>[3x]MTWHILGAGSLGSLWAARLGRAGLPVRLILRDRQRLRRYQQAGGLSLVEDGQASLYPIAAETPDGGQPIQRLLLACKAYDAEEAASSVAHRLAGNAELLLLQNGLGSQQAVAARLPRSRCLFASSTEGAFRDGDFRVVFAGRGHTWLGDPRDTNAPAWLTQLSQAG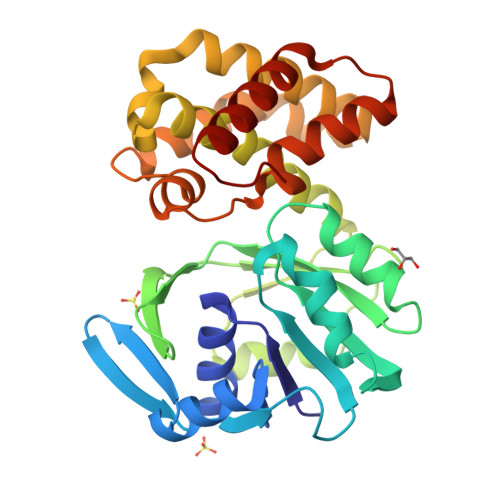IPHSWSDDILERLWRKLALNCAINPLTVLHDCRNGGLRQHPEEIAALCDELGQLLHASGYDAAARSLLEDVRAVIDATAANYSSMHQDVTRGRRTEIGYLLGYACQHGQRLGLPLPRLGTLLARLQAHLRQRGLPDR[(4R)-4-methylazepan-1-yl](1,3-thiazol-4-yl)methanone | C11 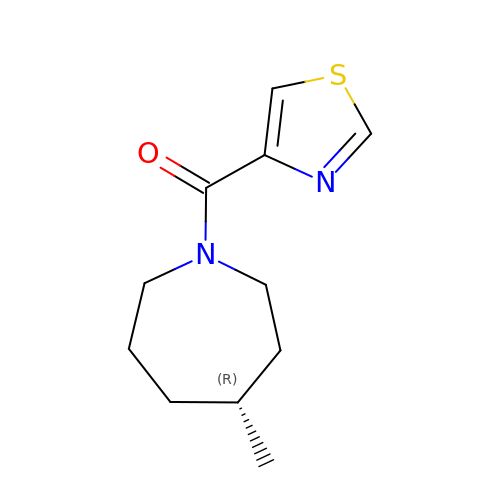H16 N2 O S | ORSJIQSXTAJDMZ-SECBINFHSA-N>[4x]MEEKAKSIDQATLQLLDKAKQDGVETVWDRKADMKVQCGFGSAGVCCRNCSMGPCRVSPVPGKGVERGICGATADVIVSRNFARMVAAGTAAHSDHGRSIALSLYHTSKDGDIKVKDENKLKEVAKSFNVETEGRDIYDIAHDVAKEGLSNYGKQLGEVTLPPSLPEKRKELWRKLGVYPRAVDREIAAVMHSTHIGCNADAEAMIKMSMRCSLTDGWMGSFMGTEFSDIMFGTPHSIDTEANLGVLEKNSVNVVLHGHEPLLSEMVVEAASDPELVELAKSVGADGINLCGMCCTGNEVSMRHGIKIAGNFMQQELAVVTGAVDGLIVDVQCIMPALAKLSKSYHTKFITTSPKAHITDSIYMEFDEENPLDSAKKILKEAILNFKNRDQSKVMIPELKCKAILGYSVEEIINKLDKVVNTQ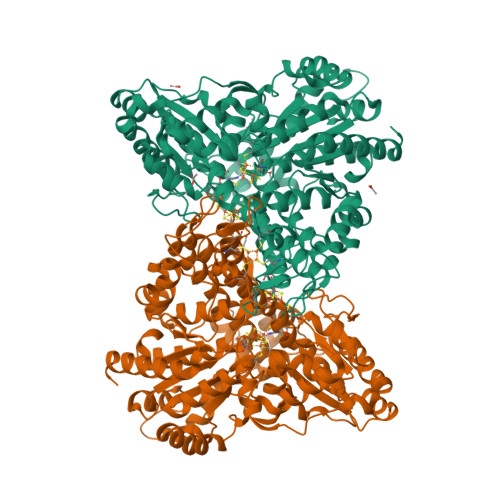IGPMQTVKPLADVLVSGVLRGAAAVVGCNNPKVVQDSAHIETIKGLIKNDVIVVVTGCAAQAAAKYGLLQKEAAEKYAGPGLATVCKLVDIPPVLHMGSCVDISRILDLVGRVANLLGVDMSDLPVAGVAPEWMSEKAVAIGTYVVTSGIDTWLGVAPPVTGGPEVVDILTNKMEDWVGAKFFIETDPHKAVEQIVNRMNEKRKKLGI>[2x]HGSPVDICTAKPRDIPMNPMCIYRSPEKKATEDEGSEQKIPEATNRRVWELSKANSRFATTFYQHLADSKNDNDNIFLSPLSIS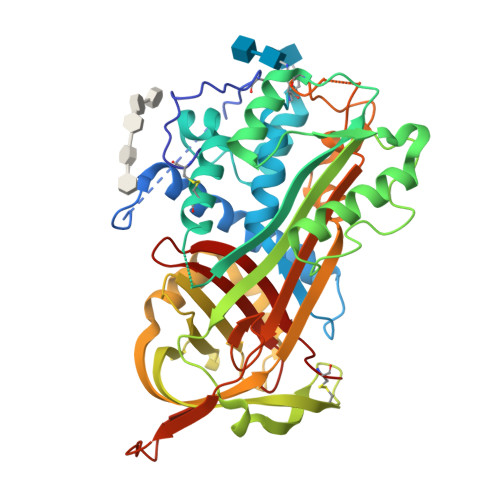TAFAMTKLGACNDTLQQLMEVFKFDTISEKTSDQIHFFFAKLNCRLYRKANKSSKLVSANRLFGDKSLTFNETYQDISELVYGAKLQPLDFKENAEQSRAAINKWVSNKTEGRITDVIPSEAINELTVLVLVNTIYFKGLWKSKFSPENTRKELFYKADGESCSASMMYQEGKFRYRRVAEGTQVLELPFKGDDITMVLILPKPEKSLAKVEKELTPEVLQEWLDELEEMMLVVHMPRFRIEDGFSLKEQLQDMGLVDLFSPEKSKLPGIVAEGRDDLYVSDAFHKAFLEVNEEGSEAAASTAVVIAGRSLNPNRVTFKANRPFLVFIREVPLNTIIFMGRVANPCVK>[8x]FASLSRFVETLVVADDKMAAFHGAGLKRYLLTVMAAAAKAFKHPSIRNPVSLVVTRLVIL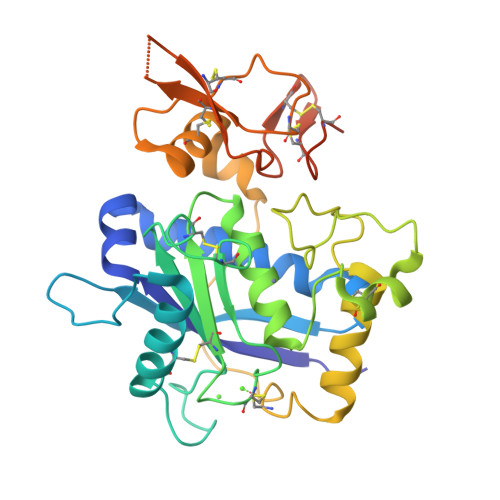GSGEEGPQVGPSAAQTLRSFCAWQRGLNTPEDSDPDHFDTAILFTRQDLCGVSTCDTLGMADVGTVCDPARSCAIVEDDGLQSAFTAAHQLGHVFNMLHDNSKPCISLNGPLSTSRHVMAPVMAHVDPEEPWSPCSARFITDFLDNGYGHCLLDKPEAPLHLPVTFPGKDYDADRQCQLTFGPDSRHCPQLPPPCAALWCSGHLNGHAMCQTKHSPWADGTPCGPAQACMGGRCLHMDQLQDFNIPQADYKDDDDK> MALKDDAVLIAARGYVYTAAVGTAAPTPSQLKLIDLEHPE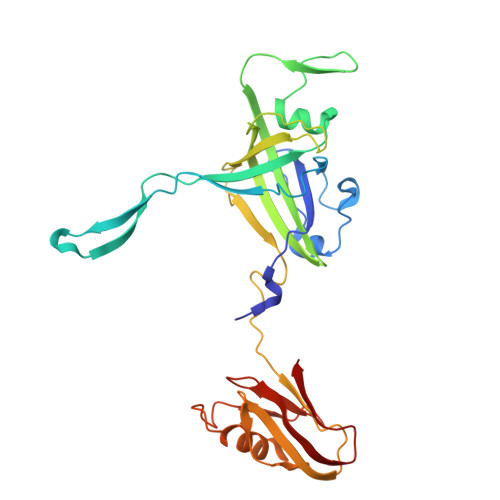AWDRTGWDLVGHTSEDDLPEFGFDGGDSEVRGSWQKKKLREVETEEIADYVVINLTQFDETALELYFGPNQSATPGIFGVKSGSVVNERALLIVIVDNDVRLGFHARKASLKREDAISLATDEFGALPVRATFLDYQSYNLYEWIEEDWFNAVDAPVVYLLDLGGATGGDYTLLVGGKSTGDIAYNANASAIKTAIGAVDDGVAESAWTVTADGSDFEISGPLAVALGVDSTTGGSGVTVDVV>SKSWGKFIEEEEAEMASRRNLMIVDGTNLGFRFKHNNSKKPFASSYVSTIQSLAKSYSARTTIVLGDKGKSVFRLEHLPEYKGNRDEKYAQRTEEEKALDEQFFEYLKDAFELCKTTFPTFTIRGVEADDMAAYIVKLIGHLYDHVWLISTDGDWDTLLTDKVSRFSFTTRREYHLRDMYEHHNVDDVEQFISLKAIMGD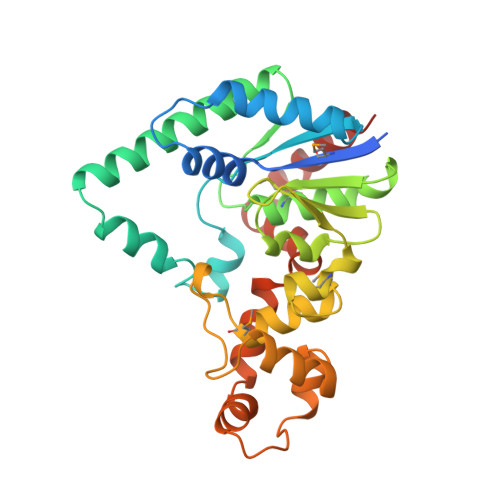LGDNIRGVEGIGAKRGYNIIREFGNVLDIIDQLPLPGKQKYIQNLNASEELLFRNLILVDLPTYCVDAIAAVGQDVLDKFTKDILEIAEQ[2x]> MSLSTPLQGIKVLDFTGVQSGPSCTQMLAWFGADVIKIERPGVGDVTRHQLRDIPDIDALYFTMLNSNKRSIELNTKTAEGKEVMEKLIREADILVENFHPGAIDHMGFTWEHIQEINPRLIFGSIKGFDECSPYVNVKAYENVAQAAGGAASTTGFWDGPPLVSAAALGDSNTGMHLLIGLLAALLHREKTGRGQRVTMSMQDAVLN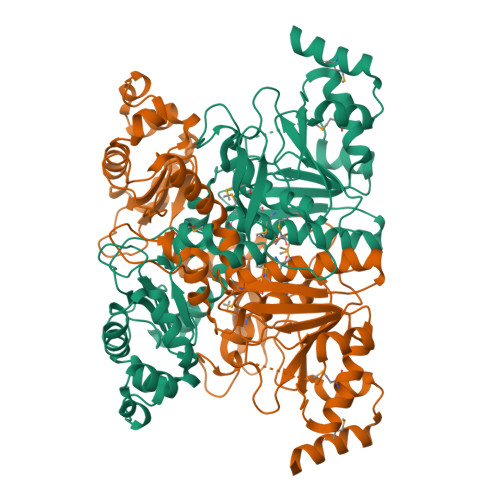LCRVKLRDQQRLDKLGYLEEYPQYPNGTFGDAVPRGGNAGGGGQPGWILKCKGWETDPNAYIYFTIQEQNWENTCKAIGKPEWITDPAYSTAHARQPHIFDIFAEIEKYTVTIDKHEAVAYLTQFDIPCAPVLSMKEISLDPSLRQSGSVVEVEQPLRGKYLTVGCPMKFSAFTPDIKAAPLLGEHTAAVLQELGYSDDEIAAMKQNHAIEGGSHHHHHH> MNIKKEFIKVISMSCLVTAITLSGPVFIPLVQGAGGHGDVGMHVKEKEKNKDENKRKDEERNKTQEEHLKEIMKHIVKIEVKGEEAVKKEAAEKLLEKVPSDVLEMYKAIGGKIYIVDGDITKHISLEALSEDKKKIKDIYGKDALLHEHYVYAKEGYEPVLVIQSSEDYVENTEKALNVYYEIGKILSRDILSKINQPYQKFLDVLNTIKNASDSDGQDLLFTNQLKEHPTDFSVEFLEQNSNEVQEVFAKAFAYYIEPQHRDVLQLYAPEAFNYMDKFNEQEINLSLEELKDQRMLARYEKWEKIKQHYQHWSDSLSEEGRGLLKKLQIPIEPKKDDIIHSLSQEEKELLKRIQIDSSDFLSTEEKEFLKKLQIDIRDSLSEEEKELLNRIQVD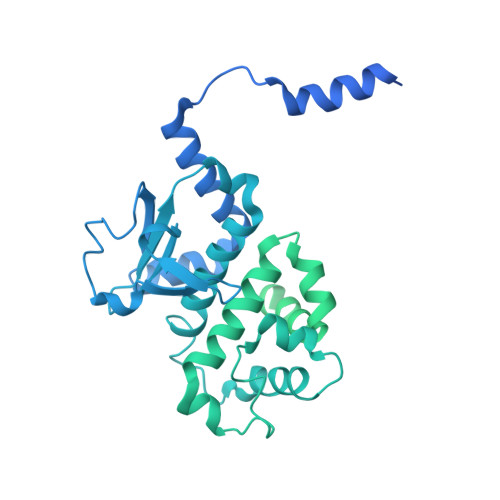SSNPLSEKEKEFLKKLKLDIQPYDINQRLQDTGGLIDSPSINLDVRKQYKRDIQNIDALLHQSIGSTLYNKIYLYENMNINNLTATLGADLVDSTDNTKINRGIFNEFKKNFKYSISSNYMIVDINERPALDNERLKWRIQLSPDTRAGYLENGKLILQRNIGLEIKDVQIIKQSEKEYIRIDAKVVPKSKIDTKIQEAQLNINQEWNKALGLPKYTKLITFNVHNRYASNIVESAYLILNEWKNNIQSDLIKKVTNYLVDGNGRFVFTDITLPNIAEQYTHQDEIYEQVHSKGLYVPESRSILLHGPSKGVELRNDSEGFIHEFGHAVDDYAGYLLDKNQSDLVTNSKKFIDIFKEEGSNLTSYGRTNEAEFFAEAFRLMHSTDHAERLKVQKNAPKTFQFINDQIKFIINS> SEGEADLYLDQYNFTTTAAIVSSVDRKIFVLLRDGRMLFGVLRTFDQYANLILQDCVERIYFSEENKYAEEDRGIFMIRGENVVMLGEVDIDKEDQPLEAMERIPFKEAWLTKQ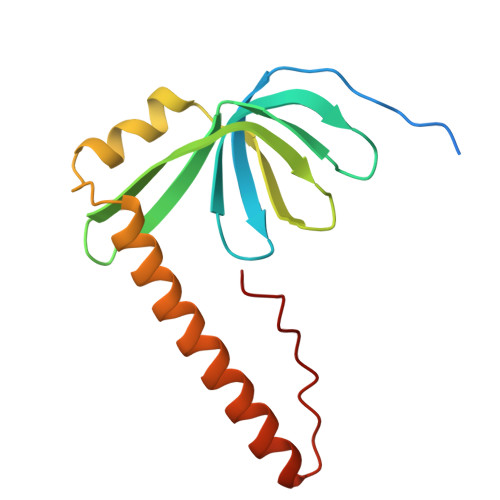KNDEKRFKEETHKGKKMARHGIVYDFHKSDMY> ADKELKFLVVDDFSTMRRIVRNLLKELGFNNVEEAEDGVDALNKLQAGGYGFVISDWNMPNMDGLELLKTIRADGAMSALPVLMVTAE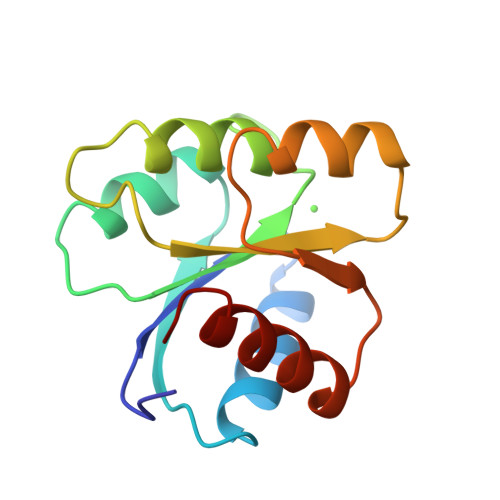AKKENIIAAAQAGASGWVVKPFTAATLEEKLNKIFEKLGM> MFKAQATFSRYSAAVSLLLLFSGAAQAAPQSITTLPLQPDGENRWRLPAGEYQGQFTIEQPMQLRCEPGAVIQSQGQGSSLLISAPDVLVEGCTLYEWGSDLTAMDSAVFILPAAERAQISNNRMRGPGFGVFVDGTRDVQVIGNEIDGDAGVRSQDRGNGIHLFAVSGARVLHNHVRNARDGIYIDTSNGNHLEGNVIEDVRYGVHYMFANENSLIDNVTRRTRTGYALMQSRKLTVTGNRSEQDQNYGILMNYITYSTITGNFVSDVQRGDTGGDSMISGGEGKALFIYNSLFNTIENNHFEKSSLGIHLTAGSEDNRISGNAFVGNQQQVKYVASRTQEWSVDGRGNYWSDYLGWDRNNDGLGDIAYEPNDNVDRLLWLYPQVRLLMNSPSIEVLRWVQRAFPVIKSPGVQDSHPLMKLPTEKLLTEKQEPTS;>[2x]MNAVEIQGVSQRYGSMTVLHDLNLNLGEGEVLGLFGHNGAGKTTSMKLILGLLSPSEGQVKVLGRAPNDPQVRRQLGYLPENVTFYPQLSGRETLRHFARLKGAALTQVDELLEQVGLA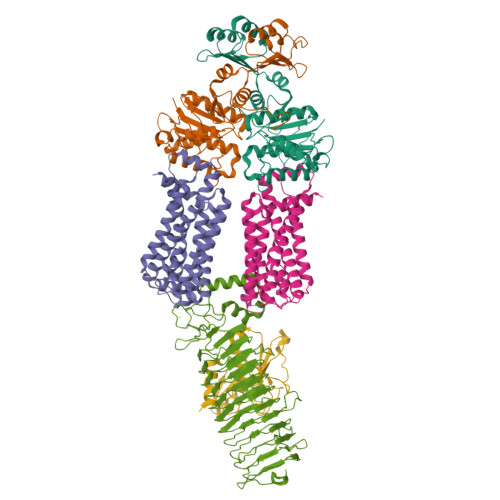HAADRRVKTYSKGMRQRLGLAQALLGEPRLLLLDEPTVGLDPIATQDLYLLIDRLRQRGTSIILCSHVLPGVEAHINRAAILAKGCLQAVGSLSQLRAEAGLPVRIRASGISERDSWLQRWTDAGHSARGLSESSIEVVAVNGHKLVLLRQLLGEGEPEDIEIHQPSLEDLYRYYMERAGDVRAQEGRL;> MNALHRIGAGTLLAVLLAFGLTGCGEKEEVQQSLEPVAFHDSDECHVCGMIITDFPGPKGQAVEKRGVKKFCSTAEMLGWWLQPENRLLDAKLYVHDMGRSVWEKPDDGHLIDATSAYYVVGTSLKGAMGASLASFAEEQDAKALAGMHGGRVLRFEEIDQALLQEAASMQHGGMHDHAPNGAHNAHAGHWSHPQFEK;>[2x]MNQVWNIARKELSDGLRNRWLLAISLLFAVLAVGIAWLGAAASGQLGFTSIPATIASLASLATFLMPLIALLLAYDAIVGEDEGGTLMLLLTYPLGRGQILLGKFVGHGLILALAVLIGFGCAALAIALLVEGVELGMLFWAFGRFMISSTLLGWVFLAFAYVLSGKVNEKSSAAGLALGVWFLFVLVFDLVLLALLVLSEGKFNPELLPWLLLLNPTDIYRLINLSGFEGSGSAMGVLSLGADLPVPAAVLWLCLLAWIGVSLLLAYAIFRRRLT> MLDLLRLQLTTFIMNDVPTPYACYFQDSATPNQEGILELHDNIMFYLLVILGLVSWMLYTIVMTYSKNPIAYKYIKHGQTIEVIWTIFPAVILLII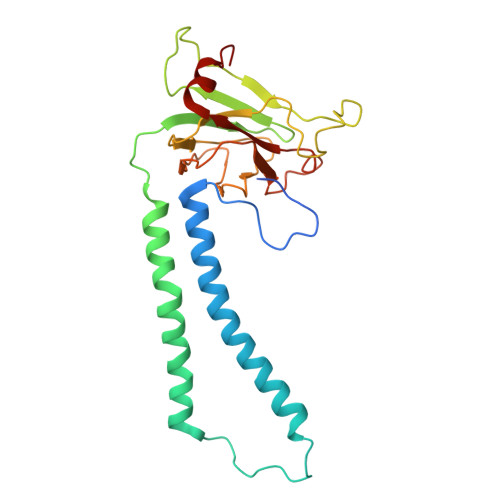AFPSFILLYLCDEVISPAMTIKAIGYQWYWKYEYSDFINDSGETVEFESYVIPDELLEEGQLRLLDTDTSMVVPVDTHIRFVVTAADVIHDFAIPSLGIKVDATPGRLNQVSALIQREGVFYGACSELCGTGHANMPIKIEAVSLPKFLEWLNEQ>[4x]QPYNPCKPQEVIDTKCMGP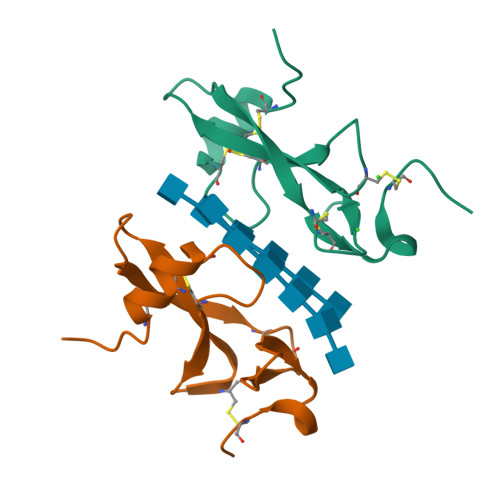KDCLYPNPDSCTTYIQCVPLDEVGNAKPVVKPCPKGLQWNDNVGKKWCDYPNLSTCPVKT> MDGSRGTAPGGDDLRGDRRDSYQGEDREDSHLLGALEDGNHQQSQGHGGGSGFYHHNVNSSSASVLEGVEMAHDELFAGPVAESVPTSVSAFSHRHGRAESVASFSFYHEQDDQREELEAPPGSLGARLSIDDLDELPFEEEGLSESEMPEQLDTFGIDLEWGSMNNGYPLIRRSSTHSQFSAHHRLLRRESGVSAASGYTGGRSSQKMRLDNDDLTIAISGFITNRIGFAIYIVLCVLTGGIAWLFLRWYPKYYVKLVGCATPFRDCQWVVIEDHFNKMTILSIRVKPYNRPLSTVFGTPSRATSWPLAQDPDPVLRELRSITYCYYKFYYHPVLDKFFCCNGWKDPQWNSMQNARSGLHGDEKAHREAVFGPNSIDVDEQSILQLLVSEILTPFYAFQVFSLILWLCDEYYYYAAAILLISAGSIITSLLETKETRRRLREMSRFECEVRVFRGGFWRTFPSSDLVPGDVYEVSDPSLTQIPADSLLLTGDCIVNESMLTGESVAVSKTPATNETLAKLNPAASTFSHDVDKHFLYCGTKLIRARQRLADTDEAAAVALVVRTGFNTTRGALVRSMLVPKPSKFKFYEDSFRYLKVMGCLAGLAFIVSLVNFIRLKLHWTLILLRALDLLTIVVPPALPATLTIGTSFAVQRLKGKKIFCTSPQRVNVGGKIDLMCFDKTGTLTEEGLDVLGIRVASRVSNRFTELLTNVDDLTWSCDSVSNGDEVKPADHVDGSSLKKDKTKPLDPYRAALYVMASCHSLRIVDGVAVGDPLEVKMFEFTGWSYEEGFIAGEVISTEGRGDISPSIARPPRYMTSQEMSIGEAPPAVGVLRAFDFNPLLRRSSVIARVVGNSGGYALVKGSPECMPEICRPETLPSDFDELLSYYTHAGYRVIACATKRIPKLNLVSVNRMTRDEVESGLDFVGFIIFENKLKPTTTSVIKELLSSNIGTVMITGDNIRTAVSVARQCGIIEEHAHCYMPRFIEGNADDCNAKLRWESINNPALELDPWTLLPMPVPPQTDASLPYDVSNIRNYAIAVTGDVFRWIVDHAPTDVLHRMLVLGKVYARMSPDEKQELVKKFQSIDYSCGFCGDGANDCAALKAADVGISLSEAEASVAAPFTSQIFDIRCVPEVIREGRASLVTSFSCFKYMSLYSFIQFTSVSFLYVSASNLGDFQFLYIDLMLILPIAVFMSWAGPHSKLCAKRPVSDLVSRKVLVPLLSHVFVCVMIQALAWVAVRQQPWYIPPIVDTEKSNIENSENTTLFFASCFEYILSGVVLNAGRPFRQSPLETWPFLSAVAVTLIATLLMLLVPPYWLFEFMQLTWMSWTFKITLIAFGFVYFLIAWTGEHYLFLWLARFLGRMRQRLFKQPKQRKLYKIVKEKLVFENLYFQ

P-type ATPases form a large membrane protein superfamily that couples ATP hydrolysis to the transport of cargo across biological membranes. In human cells, P5B-ATPases execute the active export of physiologically important polyamines such as spermine from lysosomes to the cytosol, a function linked to a palette of disorders. Here we describe a series of cryo-electron microscopy structures of a yeast homolog of human ATP13A2-5, Ypk9, determined at resolutions reaching 3.4 Å, and depicting three separate transport cycle intermediates, including spermine-bound conformations. Ypk9 exhibits ten TM helices and a soluble N-terminal domain (NTD) in close proximity to the membrane, perhaps involved in lipid regulation.

Next, additional structures were determined, all in the presence of SPM, and using N- or C-terminally linked GFP protein. We exploited conditions in the presence again of BeF3− (yielding a structure at 3.7 Å resolution overall, denoted E2P*), or without a similar compound (3.5 Å, E2.PiSPM). Structural analyses to SERCA and ATP11C-CDC50A suggest the SPM-structures are indeed caught in separate E2P and E2.Pi configurations, with the E2.PiSPM structure indicating the presence of cargo is sufficient to stabilize an E2.Pi state. While the E2.Pi structures are highly similar, distinctions are identified between the two recovered E2P states (see further below). Spermine uptake is accomplished through an electronegative cleft lined by transmembrane segments 2, 4 and 6. The cleft harbors an additional, elongated density compatible with the presence of SPM. Equivalently, completion of cargo-binding is linked to the proceeding E2.Pi state, where SPM is accommodated in a cavity on the luminal side, coordinated by conserved acidic and hydrophobic residues, including the conserved VPPALP motif. As such, the composition of the cavity also allows binding of shorter physiological polyamines, e.g., SPD and putrescine, in a similar manner. Indeed, the NTD-domain is displaced between the E2P and E2.Pi structures.> MGVKTFQFPFAEQLEKVAEQFPTFQILNEEGEVVNEEAMPELSDEQLKELMRRMVYTRILDQRSISLNRQGRLGFYAPTAGQEASQIASHFALEKEDFILPGYRDVPQIIWHGLPLYQAFLFSRGHFHGNQIPEGVNVLPPQIIIGAQYIQAAGVALGLKMRGKKAVAITYTGDGGTSQGDFYEGINFAGAFKAPAIFVVQNNRFAISTPVEKQTVAKTLAQKAVAAGIPGIQVDGMDPLAVYAAVKAARERAINGEGPTLIETLCFRYGPHTMSGDDPTRYRSKELENEWAKKDPLVRFRKFLEAKGLWSEEEENNVIEQAKEEIKEAIKKADETPKQKVTDLISIMFEELPF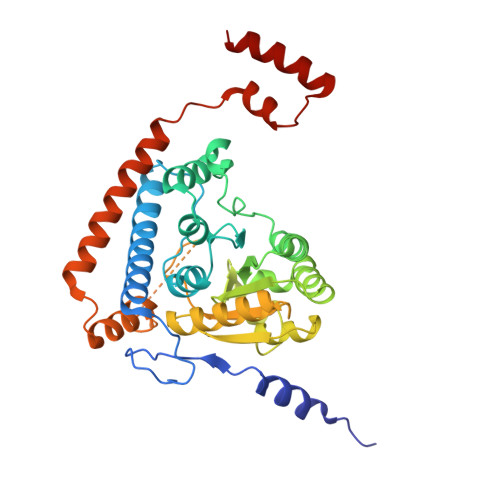NLKEQYEIYKEKESK Inteins catalyze their removal from a host protein through protein splicing. The HINT domain catalyzes the protein splicing reaction, whereas HEN domains often function independently of the HINT domain. In this study, we elucidated crystal structures of HEN-associated archaeal inteins inserted at the same insertion site (VMA-b), which is located within the A subunit P-loop of the vascular-type ATP synthase (VMA) from Thermococcus litoralis (Tli) and Pyrococcus horikoshii (Pho). The two three-dimensional structures highlighted a modular architecture consisting of HINT, HEN, and an accessory domain (ACD).

The VMA intein from P. horikoshii (PhoVMA) consists of 376 amino acids, which is considerably smaller than canonical HEN-associated inteins, e.g., SceVMA consisting of 454 residues but more similar to the size of the TFIIB intein from Methanococcus jannaschii (MjaTFIIB, 335 residues). The sequence alignment of the archaeal inteins also suggests that PhoVMA intein lacks homing endonuclease activity due to the absence of the active site residues in Blocks C and E. To prevent self-cleavages during protein production, we expressed both inteins in E. coli with alanine substitutions of the catalytic cysteines 1 (Cys1). We solved the crystal structure of the PhoVMA intein at the 2.5 Å-resolution. The crystal structure of PhoVMA intein revealed the typical HINT domain of thermophilic inteins, which contains a β-strand insertion and the HEN domain structure. As expected from the primary structure, the PhoVMA intein lacks the presumed HEN active site residues in both usually conserved LAGLIDADG helices (Blocks C and E). It shows a partial truncation in Block E, hypothetically indicating progressive HEN degeneration. As for the nested HEN domains, the deletion in Block E in the PhoVMA intein causes a truncation of the second LAGLIDADG helix by one turn, thereby removing one of the catalytic aspartate residues. The primary structures and the three-dimensional crystal structures of the VMA inteins suggest that the HEN activity of PhoVMA intein has most likely degenerated during evolution and is inactive due to the lack of active site aspartate residues. The PhoVMAΔHEN intein still retained the protein splicing activity, indicating that the HINT domain of PhoVMA intein is functionally independent of the nested HEN domain without having developed a mutualism.

> SGKAVDGDTLVLTKEFGLIKIKELYEKLDGKGRKIVEGNEEWTELEKPITVYGYKDGKIVEIKATHVYKGVSSGMVEIRTRTGRKIKVTPIHRLFTGRVTKDGLILKEVMAMHVKPGDRIAVVKKIDGGEYIKLDSSNVGEIKVPEILNEELAEFLGYLMANGTLKSGIIEIYCDDESLLERVNSLSLKLFGVGGRIVQKVDGKALVIQSKPLVDVLRRLGVPEDKKVENWKVPRELLLSPSNVVRAFVNAYIKGKEEVEITLASEEGAYELSYLFAKLGIYVTISKSGEYYKVRVSRRGNLDTIPVEVNGMPKVLPYEDFRKFAKSIGLEEVAENHLQHIIFDEVIDVRYIPEPQEVYDVTTETHNFVGGNMPTLLHN>MASMTGGQQMGRDEAGITGTWYNQLGSTFIVTAGADGALTGTYESAVGNAESRYVLTGRYDSAPATDGSGTALGWTVAWKNNYRNAHSATTWSGQYVGGAEARINTQWLLTSGTTEANAWASTYVGHDTFTKV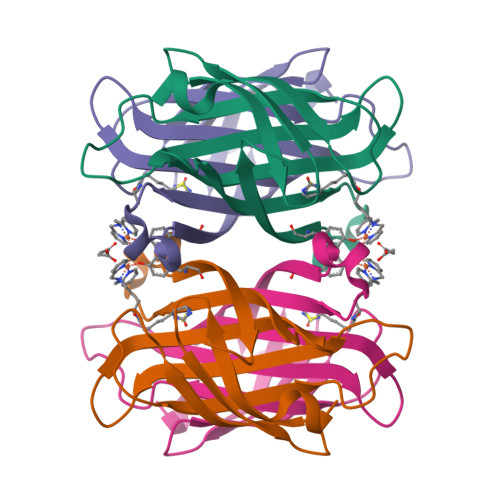KPSAASIDAAKKAGVNNGNPLDAVQQ[4x]>[4x]GAMAIRTSELLKRPPVSLPETATIREVATELAKNRVGLAVLTARDNPKRPVAVVSERDILRAVAQRLDLDGPAMPIANSPIT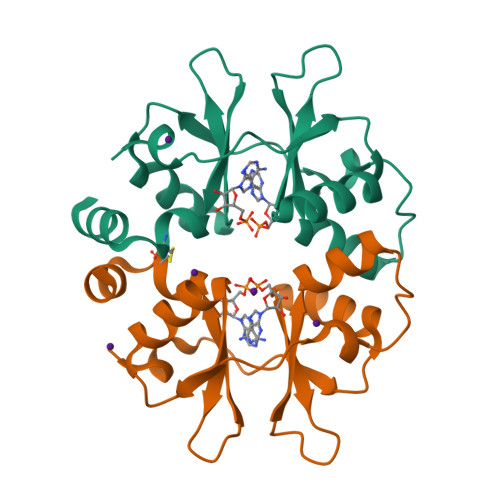VLDTDPVHVAAEKMRRHNIRHVVVVNKNGELVGVLSIRDLCFERAILLELATAEVPATP> VV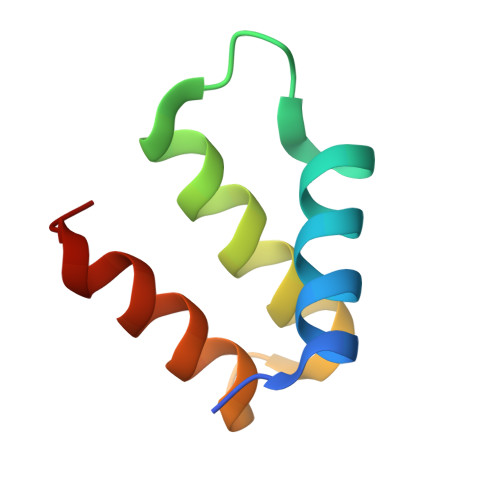GIGRDKLGKIFYRALTQYLTPTSNFSQLRAAAVQSATDLYGSTSQEVASVKQAFDAVGVK> FTLIELMIVIAIVGILAAVALPAYQDYTARAQVSEAILLAEGQKSAVTEYYLNHGKWPENNTSAGVASSPTDIKGKYVKEVEVKNGVV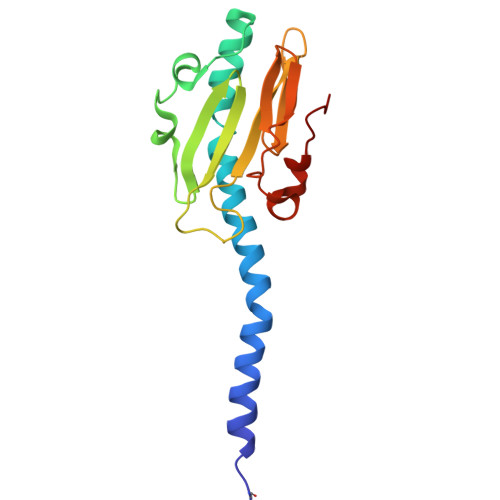TATMLSSGVNNEIKGKKLSLWARRENGSVKWFCGQPVTRTDDDTVADAKDGKEIDTKHLPSTCRDNFDAK>APVRSLNCTLRDSQQKSLVMSGPYELKALHLQGQDMEQQVVFSMSFVQGEESNDKIPVALGLKEKNLYLSCVLKDDKPTLQLESVDPKNYPKKKMEKRFVFNKIEINNKLEFESAQFPNWYISTSQAENMPVFLGGTKGGQDITDFTMQF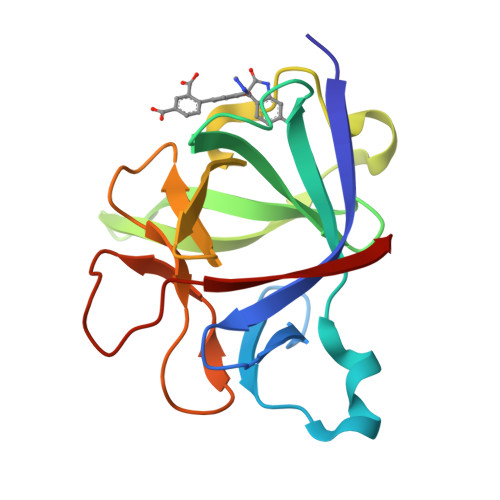VSS[2x]>QELGNANFENFIGATEGFSEIAYQFTSHILTLGYAVMLAGLLYFILTIKNVDKKFQMSNILSAVVMVSAFLLLYAQAQNWTSSFTFNEEVGRYFLDPSGDLFNNGYRYLNWLINVPMLLFQILFVVSLTTSKFSSVRNQFWFSGAMMIITGYIGQFYEVSNLTAFLVWGAISSAFFFHILWVMKKVINEGKEGISPAGQKILSNIWILFLISWTLYPGAYLMPYLTGVDGFLYSEDGVMARQLVYTIADVSSKVIYGVLLGNLAITLSKNKEL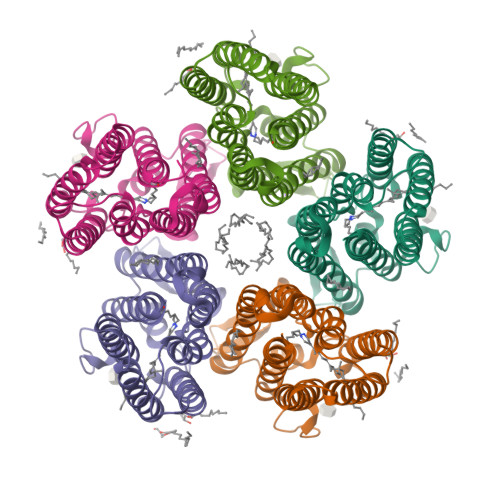[5x]>[3x]GASTLTVHVRSEEWDLMTFDA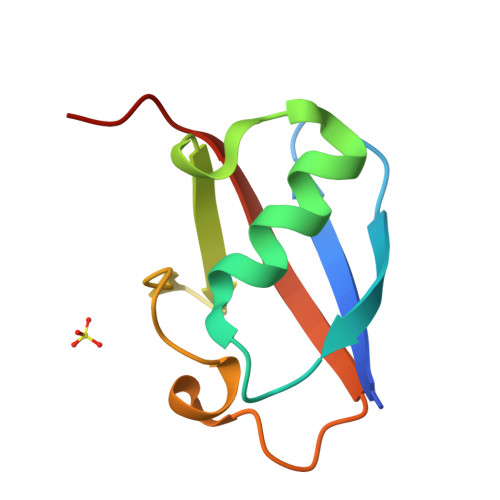NPYDSVKKIKEHVRSKTKVPVQDQVLLLGSKILKPRRSLSSYGIDKEKTIHLTLKVVKPSDE>[2x]NVLTVYSPYQSNLIRPILNEFEKQEHVKIEIKHGSTQVLLSNLHNEDFSERGDVFMGGVLSETIDHPEDFVPYQDTSVTQQLEDYRSNNKYVTSFLLMPTVIVVNSDLQGDIKIRGYQDLLQPILKGKIAYSNPNTTTTGYQHMRAIYSMHHRVSDVHQFQNHAMQLSKTSKVIEDVAKGKYYAGLSYEQDARTWKNKGYPV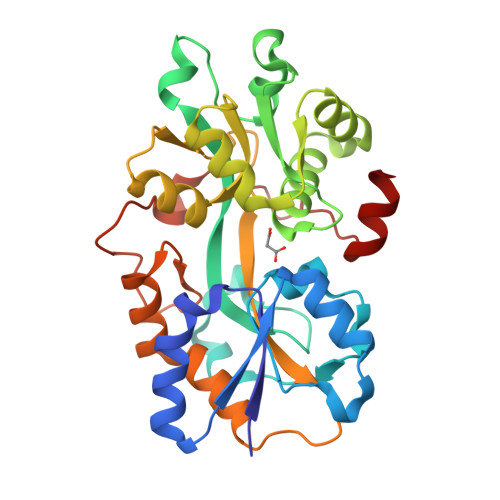SIVYPIEGTMLNVDGIALVKNAHPHPKRKKLVQYLTSRSVQQRLVAEFDAKSIRKDVSEQSDQSIENLKNIPLIPKSKLPDIPHHKFLEMIQ2-PIPERAZIN-1-YL-ANILINE | C10 H15 N3 | 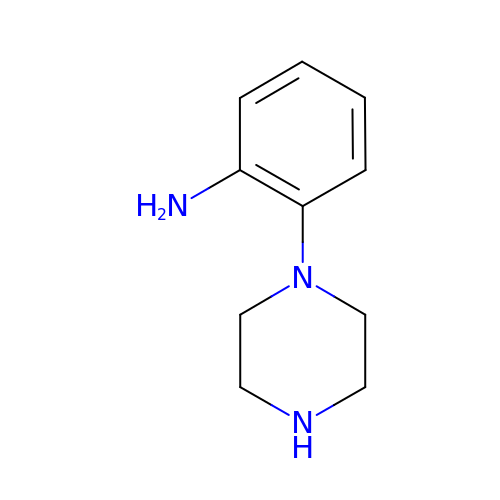TZWRXFPFRACRLO-UHFFFAOYSA-N> GTSTQTKAGSLTIVGTGIESIGQMTLQALSYIEAAAKVFYCVIDPATEAFILTKNKNCVDLYQYYDNGKSRLNTYTQMSELMVREVRKGL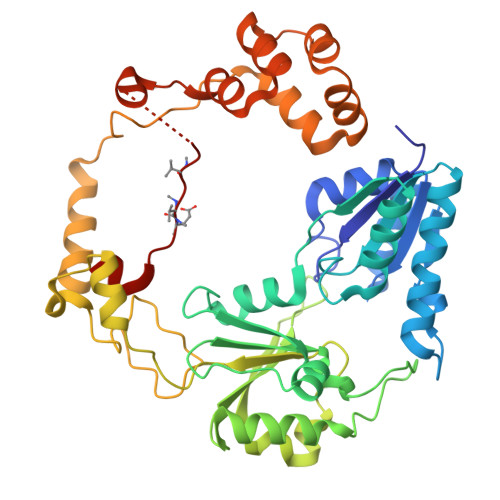DVVGVFYGHPGVFVNPSHRALAIAKSEGYRARMLPGVSAEDCLFADLCIDPSNPGCLTYEASDFLIRDRPVSIHSHLVLFQVGCVGIADFNFTGFDNNKFGVLVDRLEQEYGAEHPVVHYIAAMMPHQDPVTDKYTVAQLREPEIAKRVGGVSTFYIPPKARKASNLDIIRRLELLPAGQVPDKKARIYPANQWEPDVPEVEPYRPSDQAAIAQLADHAPPEQYQPLATSKAMSDVMTKLALDPKALADYKADHRAFAQSVPDLTPQERAALELGDSWAIRCAMKNMPSSLLDAARESGEEASQNGFPWVIVXGVIGVIGSVMSTE>[2x]MDDLTLRYFDAEMRYLREAGKAFAQAHPDRAAMLDLDKAGTPDPCVERLFEGFAFSMGRLRQKIDDDLPELTESLVSMLWPHYLRTIPSLSVVALTPRLSVMKMAETVPAGLEVTSRPVGPGNTVCRYRTTRAIPLNPLAVEKVVMTTEPDGRSVLKIGFACSELADWSQVDLHRLSLYLAAE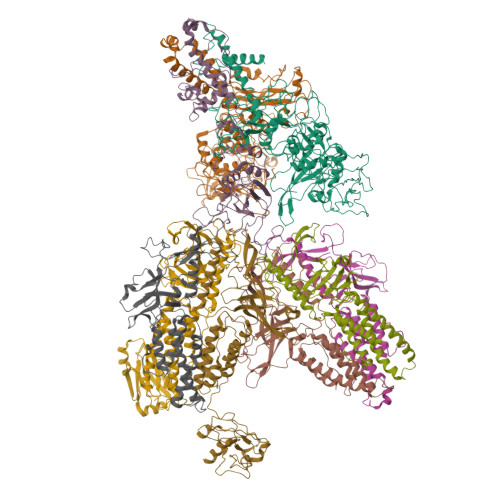APVSSTLHLMMTKRLAALYLRLPGNDERIRIDGWFSPGGFAEEDRLWPKGDSAFSGYQLLLEYFTFREKFMFVHLNGLENVSLPAGISGFDLEVVLSQPWPADLPVTDDALCLHCVPVINLFTLEADPLIINGLESEYLLRPKRLQDGYTEIYSVDAVTGSGRTGSAEYVPFTSFRHRGGMLRHDAPERYYHTRVKRGVTGMYDTWLILGGQRWEADRMPERETLSLRITGTNGQLPRRALQSTLLDRCEQVLQAPVSVRNLCKPTLPVYPPTEDRFHWRVMSHLGTGFLNMLSSAEVLRGTLALYNWRDDELNHRRLDAILAVQHHRIQRFEKGFLLRGLDVEVTLDGNGFAGEGDIHLFGEMLNRFLALYADMNQFNQLTLIVQPEGKCIRWKENHNPRLPG;> MHPVERKSQSAPARLITRYRKQLPYINFYRFCQLLEQSQPDQPPIGSGWQARQEAVRFCPYPGMGFPASEIKDAVIPEESHLPPIVHVTFMGLYGVTSPLPAHYISDIAQQREGHEAAADFLDIFSHRLITQYYRIWRKYSYPATFEAGGQDKTSQYLLGLARLGIPGCAQNIATPVSRFLALLPLMLLPGRTAEGLTSLVTLLAPGTQARVWHHDRRRIPLKTPLTMRVHHPVSLKSRPVMGDHATDVNGQVLLQLSTQTGSEVQGWLPGGHLYSDLLALLHVYLGSRLDVRLQLCVERSLLPDARLSCRPAAGSPQLGRTAVMRTQAKIATSAARVMTISLGRYQRVQEHYQRKETQENGDYRW;>[6x]MKIYRPLWEDGAFLMPQQFQQQAAWDVHLADSVARMGLAHPWGVVAAEFDDSLLPLSRLNATRLIVRFPDGTLIDTERADNLPPVCDLSTVSDRSLVDIVLALPLLNANGGNLDNGSESERPRRWKSERVNVQELAGHEQSEVAVLRHNLTLRMAHQENAAWLTCPVTRLVRDAQGQWCRDPRFIPPLLTLSASPSLMTELLELLHHLQARRQRLMSMRRENNARLADFAVADVSLFWLLNALNSAEPVLKELLDMPYRHPELLYRELARLAGSLLTFSLEHNVDAVPAYHHETPENVFPPLLSLLNRLLEASLPSRVVFIELKQKGVMWEGALHDARLREGADFWLSVRSSMPGHELQTKFPQLCKAGSPDDVSEVVNVALSGVIIRPVTHVPAAIPLRLENQYFALDLSTDAARAMLDAGRCTFYTPASLGDVKLELFAVLR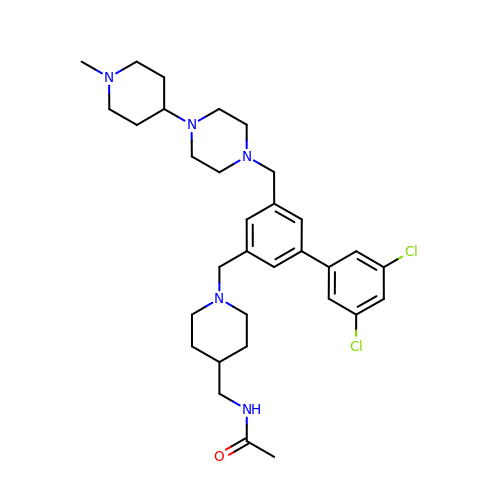~{N}-[[1-[[3-[3,5-bis(chloranyl)phenyl]-5-[[4-(1-methylpiperidin-4-yl)piperazin-1-yl]methyl]phenyl]methyl]piperidin-4-yl]methyl]ethanamide | C32 H45 Cl2 N5 O | CZHJIRYUHXUOHG-UHFFFAOYSA-N>[2x]MLKSRVILAMDKPLSYQVLKEMENELYGIKVGLPLVLDLGVDKTRELLIGLDVEEIIVDFKLADIGYIMKSIVERLSFANSFIAHSFIGVK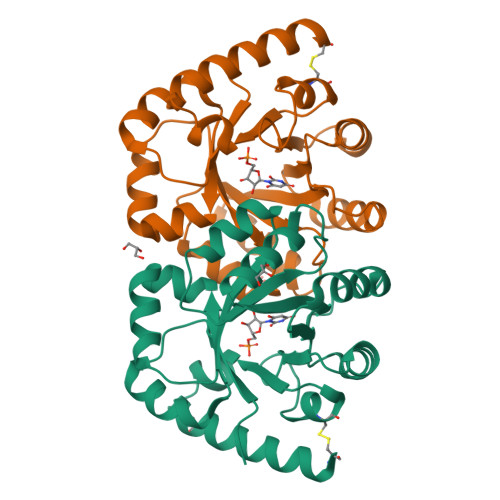GSLDELKRYLDANSKNLYLVAVMSHEGWSTLFADYIKNVIREISPKGIVVGGTKLDHITQYRRDFEKMTIVSPGMGSQGGSYGDAVCAGADYEIIGRSIYNAGNPLTALRTINKIIEDKVMKCKGAIFRKK>HPNYKLTYFNMRGRAEIIRYIFAYLDIQYEDHRIEQADWPEIKSTLPFGKIPILEVDGLTLHQSLAIARYLTKNTDLAGNTEMEQCHVDAIVDTLDDFMSCFPWAEKKQDVKEQMFNELLTYNAPHLMQDLDTYLGGREWLIGNSVTWADFYWEICSTTLLVFKPDLLDNHPRLVTLRKKVQA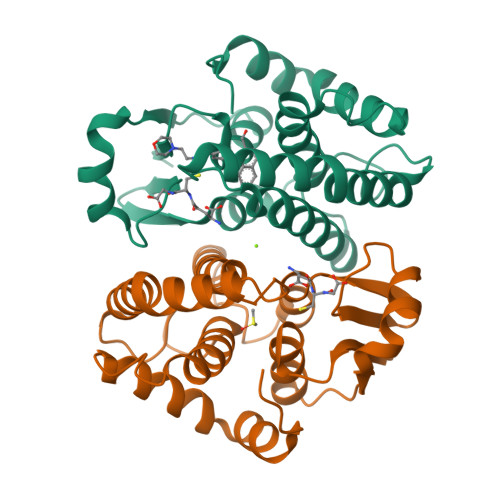IPAVANWIKRRPQTKL[2x]>[2x]GPASPDRFAVSAEAENKVREQQPHVERIFSVGVSVLPKDCPDNPHIWLQLEGPKENASRAKEYLKGLCSPELQDEIHYPPKLHCIFLGAQGFFLDCLAWSTS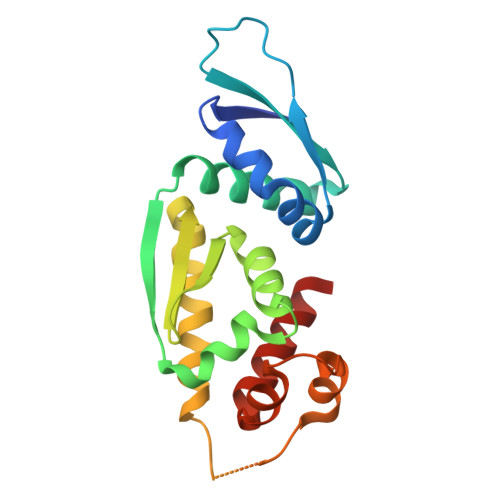AHLVPRAPGSLMISGLTEAFVMAQSRVEELAERLSWDFTPGPSSGASQCTGVLRDFSALLQSPGDAHREALLQLPLAVQEELLSLVQEASSG>MRTFARRARPPAAILFSESMQSIPLSLPLSRTAFFFDFDGTLVDLAPTPDAIQVPPDVPVLVDALRQLSHGAVAIVSGRGIDSIDAYLNLPGLPVAGLHGAERRDANGDTQRIGFDDPRLLRIERELAALVDRHPGMLLEIKGAALALHFRNAPEREGVARAAAERLVADYADAYVLQPGKMVFE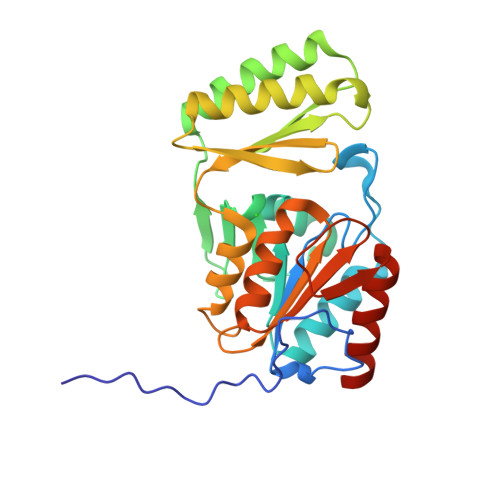IKPKGVDKGRAVAAFLNEPPFAGRMPVFAGDDLTDEQGFAVANANGGLSIKVGAGDTTARARVDSVAALRAQLARWIAAGRAPA[2x]> GAMAPIEYLLFEEPTGYAVFKVKLQQDDIGSRLKEVQEQINDFGAFTKLIELVSFAPFKGAAEALENANDISEGLVSESLKAILDLNLPKASSKKKNITLAISDKNLGPSIKEEFPYVDCISNELAQDLIRGVRLHGEKLFKGLQSGDLERAQLGLGHAYSR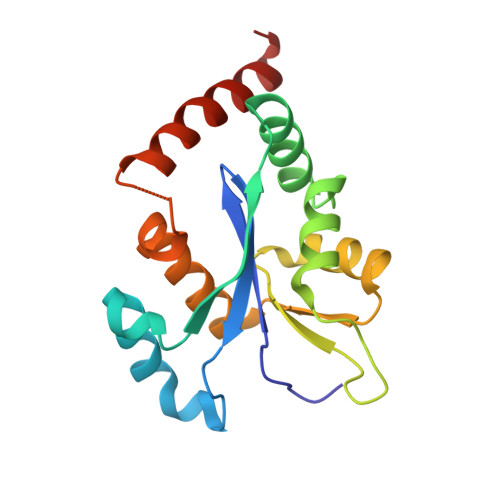AKVKFS> GSHMASGEGPALYEDPPDQKTSPSGKPATLKICSWNVDGLRAWIKKKGLDWVKEEAPDILCLQETKCSENKLPAELQELPGLSHQYWSAPSDKEGYSGVGLLSRQCPLKVSYGIGDEEHDQEGRVIVAEFDSFVLVTAYVPNAGRGLVRLEYRQRWDEAFRKFLKGLASRKPLVLCGDLNVAHEEI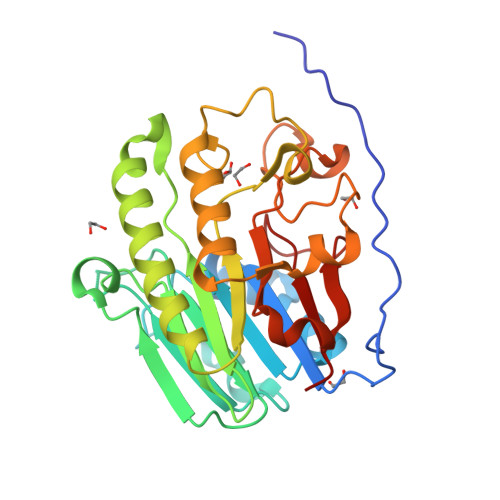DLRNPKGNKKNAGFTPQERQGFGELLQAVPLADSFRHLYPNTPYAYTFWTYMMNARSKNVGWRLDYFLLSHSLLPALCDSKIRSKALGSDHCPITLYLAL>AHDLEADVTMTGSDLVSCCYRSLAAPDLTLRDLLDIVETSQAHNARAQLTGALFYSQGVFFQWLEGRPAAVAEVMTHIQRDRRHSNVEILAEEPIAKRRFAGWHMQLSCSEADMRSLGLAESRQIVTVGRSLVADNTNIFSFDRIAAVRRFLSDVCAARTLAPDTPVEADTFALYALTEAQAGRSGRAKAVARLSDLLSTDPLGRLTEVEELLRAHAPTAADFARLFEACAERLTRALAEDRISRMQVTLAYSALQMALRRIHHLPDPQKSVGAVLVAG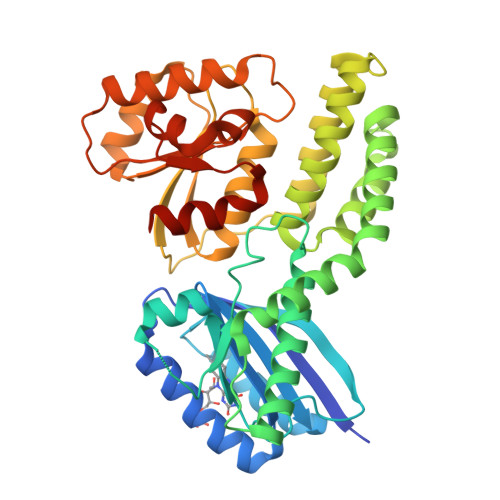VPGHKPILEAALAAEMLRAVGWSTSVVHPESVAALAARLKTSRTSTLVVAPSLLEGTEQEADTLRFVSALRARTDLPGLSILVGGRLAQLPPSKLKDSGADAGFAHLALLPAALARVASSAHHHHHH[2x]> MAEIKHYQFNVVMTCSGCSGAVNKVLTKLEPDVSKIDISLEKQLVDVYTTLPYDFIL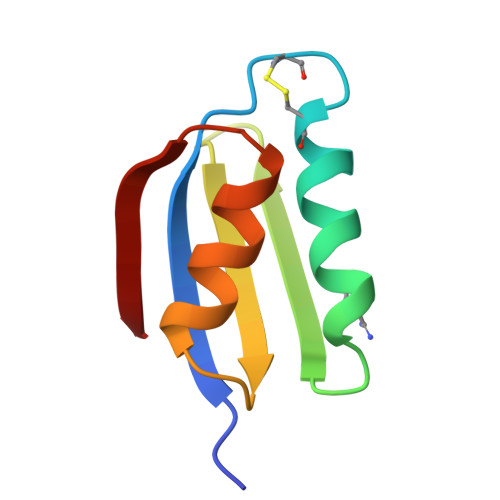EKIKKTGKEVRSGKQL>[2x]APDTSVSNKQNFSTDVIYQIFTDRFSDGNPANNPTGAAFDGSCTNLRLYCGGDWQGIINKINDGYLTGMGITAIWISQPVENIYSVINYSGVNNTAYHGYWARDFKKTNPAYGTMQDFKNLIDTAHAHNIKVIIDFAPNHTSPASSDDPSFAENGRLYDNGNLLGGYTNDTQNLFHHYGGTDFSTIENGIYKNLYDLADLNHNNSSVDVYLKDAIKMWLDLGVDGIRVDAVKHMPFGWQKSFMATINNYKPVFTFGEWFLGVNEISPEYHQFANESGMSLLDFRFAQKARQVFRDNTDNMYGLKAMLEGSEVDYAQVNDQVTFIDNHDMERFHTSNGDRRKLEQALAFTLTSRGVPAIYYGSEQYMSGGNDPDNRARLPSFSTTTTAYQVIQKLAPLRKSNPAIAYGSTHERWINNDVIIYERKFGNNVAVVAINRNMNTPASITGLVTSLPRGSYNDVLGGILNGNTLTVGAGGAASNFTLAPGGTAVWQYTTDATTPIIGNV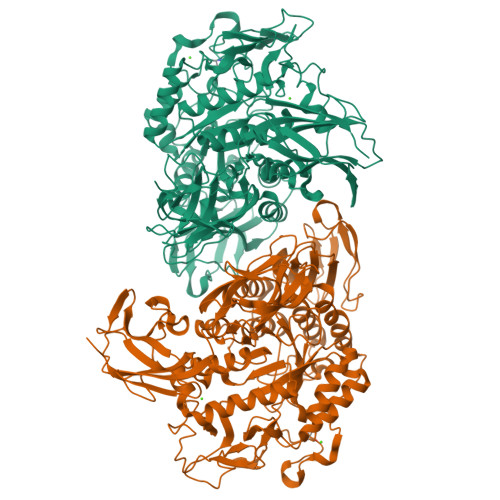GPMMAKPGVTITIDGRGFGSGKGTVYFGTTAVTGADIVAWEDTQIQVKIPAVPGGIYDIRVANAAGAASNIYDNFEVLTGDQVTVRFVINNATTALGQNVFLTGNVSELGNWDPNNAIGPMYNQVVYQYPTWYYDVSVPAGQTIEFKFLKKQGSTVTWEGGANRTFTTPTSGTATVNVNWQP>MHNGWMSTAATAQEAQGLLLQLLDPATRADPYPIYDRIRRGGPLALPEANLAVFSSFSDCDDVLRHPSSCSDRTKSTIFQRQLAAETQPRPQGPASFLFLDPPDHTRLRGLVSKAFAPRVIKRLEPEITALVDQLLDAVDGPEFNLIDNLAYPLPVAVICRLLGVPIEDEPKFSRASALLAAALDPFLALTGETSDLFDEQMKAGMWLRDYLRALIDERRRTPGEDLMSGLVAVEESGDQLTEDEIIATCNLLLIAGHETTVNLIANAALAMLRTPGQWAALAADGSRASAVIEETMRYDPPVQLVSRYAGDDLTIGTHTVPKGDT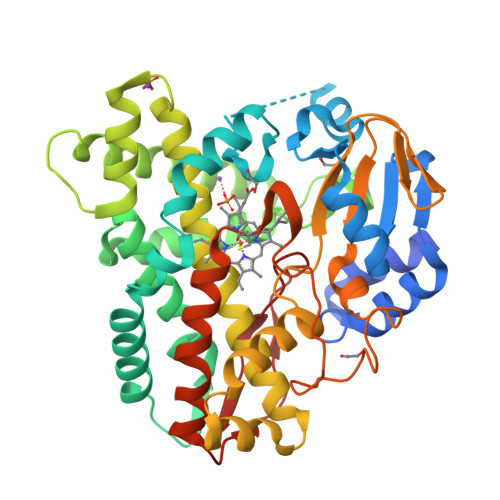MLLLLAAAHRDPTIVGAPDRFDPDRAQIRHLGFGKGAHFCLGAPLARLEATVALPALAARFPEARLSGEPEYKRNLTLRGMSTLSIAVHHHH[3x]>MKHHHHHHSAGLEVLFQGPMEDGEVNDVVHPQVRAHINSLVSALGGISIDDDGGYKLGDDALEVLRDLKKWIRFYDEKTNRMDVARCLAEANIVSTDLLHILALWTPNENSNKYKARIALACFELMVPLTWPIEKDRETMTINHHRHIPVLQLAQLGYKRAIINYDAAPILSTAVRVALPAMAMPIGERTARDQGIIKLILYFLRNIAMITPPPGVKYEGDESQISRSALIDAFSYQDIFLTLLTIASNMGEDFRTEDVIVMEIIFHLVKRVDPKGQQLGSFVSDFLDSGFNPLFSHIRKSLEREAPHVLHYHQSQFFYLVAWFLEAERARRSSFNLIASVLTQEMFIALNRALDRAYGDKDWRLLTSAMRCFTQILLTVQEMFDSGNDEDQEIADNILSRLFYEESTHDAVANIVRTYKDQGFEYLDACTELAHTFLRILEAYSKQNVDLQVRSGSADDEKMAEKTSQERKFDFKRFAARFTPQGVVDTFVTFTKYYRDLDDSQLKRAHRYFYRVAFKQEMSVMLFRLDIIHLFYNMIKGPEPLDKNSPMYKEWEELVRQILKRCIRKLEERPALFTEILFSKINSTAYYLEYGFEKQ[3x];>MTDALGIDKELNLKKKQRAPKVKLDDQRLLSEKGIPKLRKMAPRLKFKGKGHEFSDTARLLSFYQEWLDDLFPKATFLDALAMVEKAGHKTTVRNARLKWIDELRPKASFE[3x]

The Tof1–Csm3 fork protection complex has a central role in the replisome—it promotes the progression of DNA replication forks and protects them when they stall, while also enabling cohesion establishment and checkpoint responses. Additionally it has an important role in protecting stalled forks and enabling their restart, coupling the replicative helicases and polymerases, promoting fork progression, mediating the S phase checkpoint and maintaining genome stability at CAG repeats. The mammalian orthologue of Tof1–Csm3 is the Timeless–Tipin complex, which has similar functions and additionally regulates the fork in response to oxidative stress. The structure reveals that, instead of containing distinct domains, the entire complex forms an extended alpha-helical repeat protein.

Here, I present the crystal structure of the Tof1–Csm3 complex from Chaetomium thermophilum at 3.1 Å resolution. The only construct of the complex resulting in diffracting crystals was Tof1(1–728)ΔL1,2,3–Csm3(48–157). Here, three predicted disordered loops were deleted from Tof1: L1 (256–363), L2 (420–434), L3 (558–585). Tof1 begins with two helices linked by a beta-hairpin, which is then followed by eight three-helix armadillo repeats (Arm1–8). Csm3 further extends the alpha-helical repeat structure by forming a five-helix bundle which packs on the C-terminus of Tof1. However, in contrast to this domain, the helical bundle of Csm3 is flattened such that it no longer has a hydrophobic core and thus does not appear to be an independently folded structure and rather acts as a cap on the C-terminus of Tof1. The interface between the two is largely hydrophobic with some salt bridges, and consists of a large percentage of Csm3, showing why both proteins are required to stabilize each other. α25 and α26 from Arm-8 plus the following helix α27 contain all the interaction sites for Csm3. As previously noted, there is a highly conserved cleft within this interior towards the N-terminus of Tof1, lined with basic and hydrophobic residues. In our structure, the purification tag of a symmetry copy occupies this cleft. Furthermore, this interaction occurs in all three copies in the asymmetric unit despite the lack of symmetry in the packing, which suggests the cleft has a very high propensity for peptide binding.> MALLNIFDIAGSALAAQSKRLNVAASNLANADSVTGPDGQPYRAKQVVFQVDAAPGQATGGVKVASVIESQAPEKLVYEPGNPLADANGYVKMPNV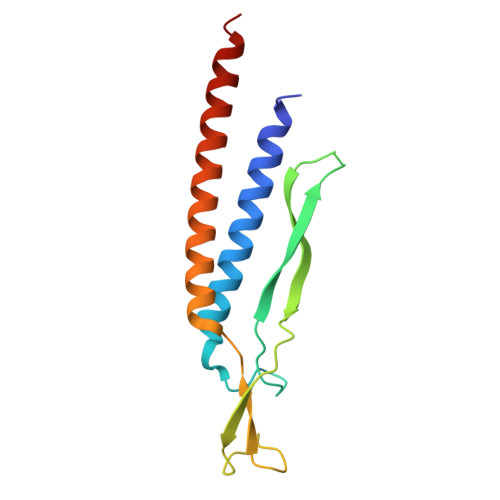DVVGEMVNTMSASRSYQANIEVLNTVKSMMLKTLTLGQ> GAHKYKKQFRYESQLQMVQVTGSSDNEYFYVDFREYEYDLKWEFPRENLEFGKVLGSGAFGKVMNATAYGISKTGVSIQVAVKMLKEKADSSEREALMSELKMMTQLGSHENIVNLLGACTL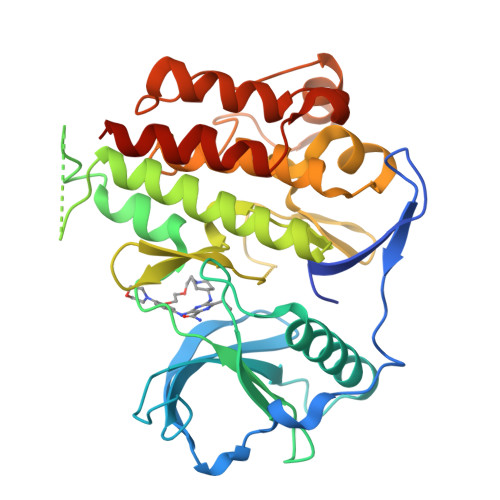SGPIYLIFEYCCYGDLLNYLRSKREKFSEDEIEYENQKRLEEEEDLNVLTFEDLLCFAYQVAKGMEFLEFKSCVHRDLAARNVLVTHGKVVKICDFGLARDIMSDSNYVVRGNARLPVKWMAPESLFEGIYTIKSDVWSYGILLWEIFSLGVNPYPGIPVDANFYKLIQNGFKMDQPFYATEEIYIIMQSCWAFDSRKRPSFPNLTSFLGCQLADAEEAMYQNV>EFARPCIPKSFGYSSVVCVCNATYCDSFDPPTFPALGTFSRYESTRSGRRMELSMGPIQANHTGTGLLLTLQPEQKFQKVKGFGGAMTDAAALNILALSPPAQNLLLKSYFSEEGIGYNIIRVPMASCDFSIRTYTYADTPDDFQLHNFSLPEEDTKLKIPLIHRALQLAQRPVSLLASPWTSPTWLKTNGAVNGKGSLKGQPGDIYHQTWARYFVKFLDAYAEHKLQFWAVTAENEPSAGLLSGYPFQCLGFTPEHQRDFIARDLGPTLANSTHHNVRLLMLDDQRLLLPHWAKVVLTDPEAAKYVHGIAVHWYLDFLAPAKATLGETHRLFPNTMLFASEACVGSKFWEQSVRLGSWDRGMQYSHSIITNLLYHVVGWTDWNLALNPEGGPNWVRNFVDSPIIVDITKDTFYKQPMFYHLGHFSKFIPEGSQRVGLVASQKNDLDAVALMHPDGSAVVVVLNRSSKDVP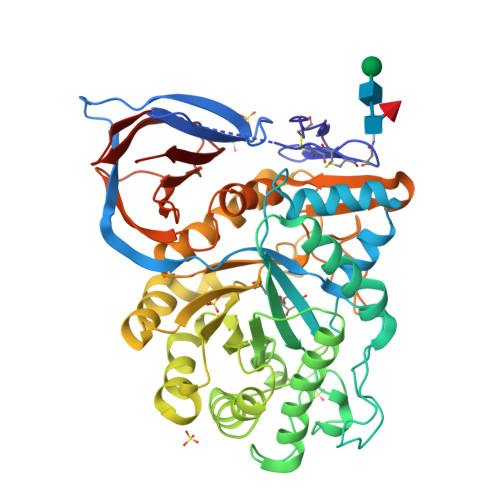LTIKDPAVGFLETISPGYSIHTYLWHRQLLVDTM[2x]>MSEIITFPQQTVVYPEINVKTLSQAVKNIWRLSHQQKSGIEIIQEKTLRISLYSRDLDEAARASVPQLQTVLRQLPPQDYFLTLTEIDTELEDPELDDETRNTLLEARSEHIRNLKKDVKGVIRSLRKEANLMASRIADVSNVVILERLESSLKEEQERKAEIQADIAQQEKNKAKLVVDRNKIIESQDVIRQYNLADMFKDYIPNISDLDKLDLANPKKELI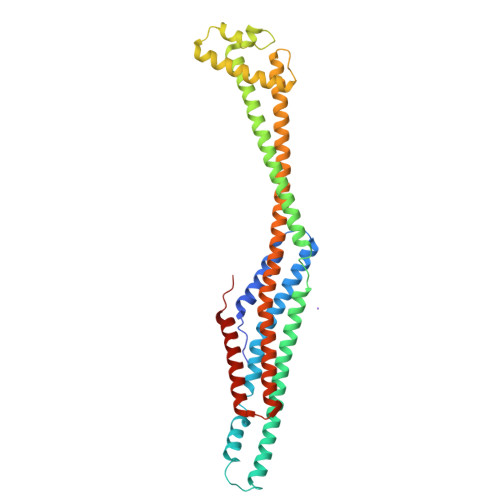KQAIKQGVEIAKKILGNISKGLKYIELADARAKLDERINQINKDCDDLKIQLKGVEQRIAGIEDVHQIDKERTTLLLQAAKLEQAWNIFAKQLQNTIDGKIDQQDLTKIIHKQLDFLDDLALQYHSMLLS[4x]>[4x]GIDPFTFENATSDAINQDMMLYIERIAKI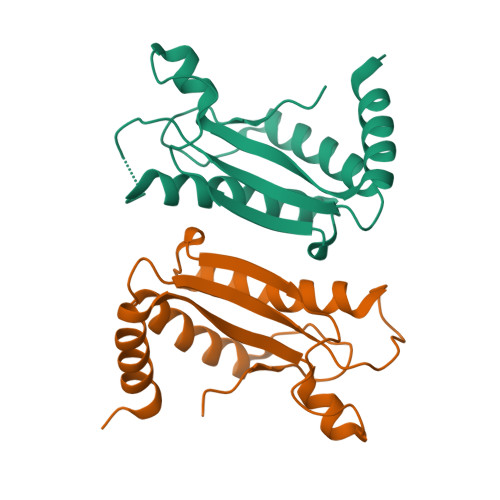IQKLPKRVHINVRGFTDDTPLVKTRFKSHYELAANRAYRVMKVLIQYGVNPNQLSFSSYGSTNPIAPNDSLENRMKNNRVEIFFSTDANDLSKIHSILDNEFNPHKQQE>[3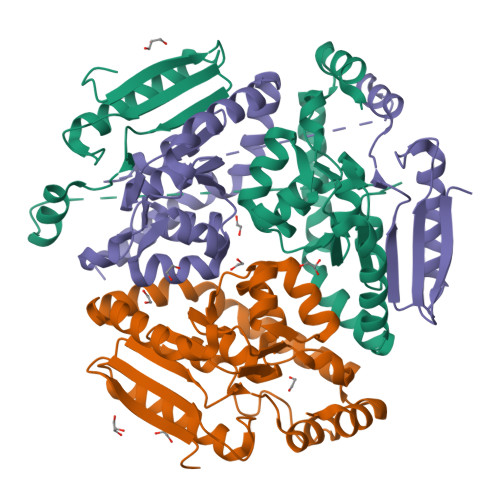x]MAHHHHHHSSGLEVLFQGPMTHSVVELIEIESAIIQVKMQDRTHKNAFSQELTDDLIQAFEYIRQNPKYKAVILTGYDNYFASGGTQEGLLRIQQGLTKFTDDNLYSLALDCEIPVIAAMQGHGIGGGFVMGLFADIVILSRESVYTANFMKYGFTPGMGATFIVPKKLGFSLAQEILLNAGSYRGADLEKRGVPFKVLPRAEVLDYAVELAQELAEKPRNSLVTLKDHLVAPLRDQLPRVIEQELMMHEKTFHHEEVKSRIKGLYGN> SDSAFSRLYT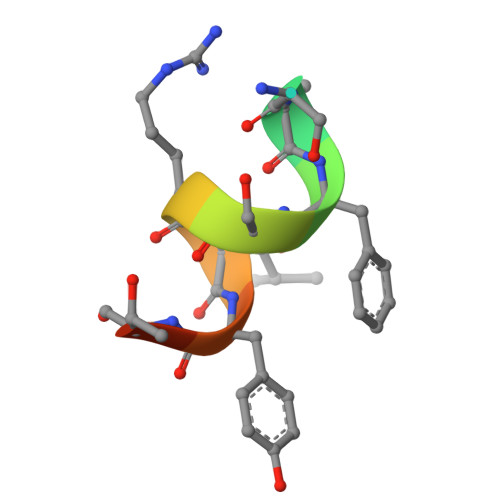RS> IPEYVDWRQKGAVTPVKNQGSCGSCWAFSAVVTIEGIIKIRTGNLNQYSEQELLDCDRRSYGCNGGYPWSALQLVAQYGIHYRNTYPYEGVQRYCRSREKGPYAAKTDGVRQVQPYNQGALLYSIANQPVSVVLQAAGKDFQLYRGGIFVGPCGNKVDHAVAAVGYGPNYILIKNSWGTGWGENGYIRIKRGTGNSYGVCGLYTSSFYPVKN;> MMSGAPSATQPATAETQHIADQVRSQLEEKYNKKFPVFKAVSFKSQVVAGTNYFIKVHVGDEDFVHLRVFQSLPHENKPLTLSNYQTNKAKHDELTY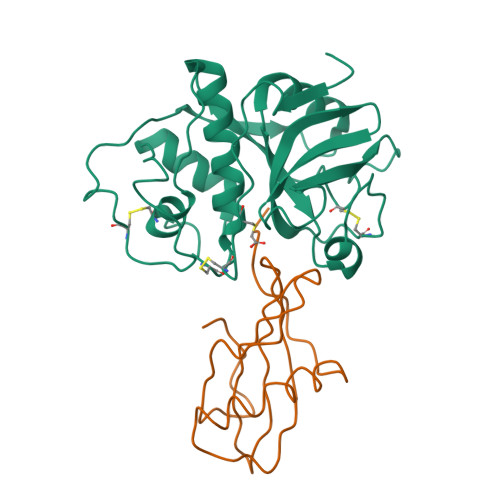F>[34x]MSATASTATQPKPLEWLNRLRANPRIPLIVAGSAAVAIVVAMVLWAKTPDYRTLFSNLSDQDGGAIVAQLTQMNIPYRFANGSGAIEVPADKVHELRLRLAQQGLPKGGAVGFELLDQEKFGISQFSEQVNYQRALEGELARTIETLGPVKSARVHLAMPKPSLFVREQKSPSASVTVTLEPGRALDEGQISAVVHLVSSAVAGLPPGNVTLVDQSGHLLTQSNTSGRDLNDAQLKFANDVESRIQRRIEAILSPIVGNGNVHAQVTAQLDFANKEQTEEHYSPNGDASKATLRSRQLNISEQVGAGYPGGVPGALSNQPAPPNEAPIATPPTNQQNAQNTPQTSTSTNSNSAGPRSTQRNETSNYEVDRTIRHTKMNVGDIERLSVAVVVNYKTLADGKPLPLTADQMKQIEDLTREAMGFSDKRGDTLNVVNSPFSAVDNTGGELPFWQQQSFIDQLLAAGRWLLVLVVAWILWRKAVRPQLTRRVEEAKAAQEQAQVRQETEEAVEVRLSKDEQLQQRRANQRLGAEVMSQRIREMSDNDPRVVALVIRQWMSNDHE;>MSNLSGTDKSVILLMTIGEDRAAEVFKHLSTREVQALSTAMANVRQISNKQLTDVLSEFEQEAEQFAALNINANEYLRSVLVKALGEERASSLLEDILETRDTTSGIETLNFMEPQSAADLIRDEHPQIIATILVHLKRSQAADILALFDERLRHDVMLRIATFGGVQLAELTEVLNGLLDGQNLKRSKMGGVRTAAEIINLMKTQQEEAVITAVREFDGELAQKIIDEMFLFENLVDVDDRSIQRLLQEVDSESLLIALKGAEPPLREKFLRNMSQRAADILRDDLANRGPVRLSQVENEQKAILLIVRRLAETGEMVIGSGEDTYV[34x];>[34x]MGDSILSQAEIDALLNGDSDTKDEPTPGIASDSDIRPYDPNTQRRVV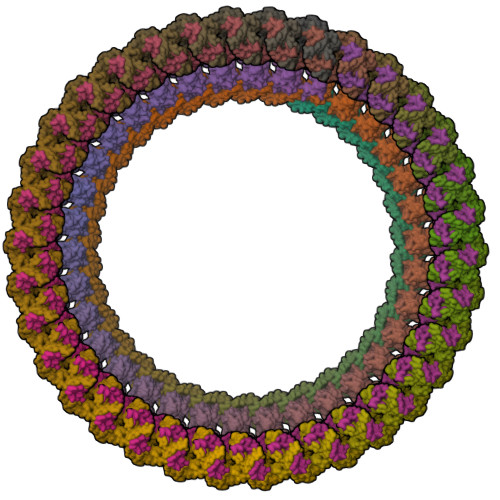RERLQALEIINERFARQFRMGLFNLLRRSPDITVGAIRIQPYHEFARNLPVPTNLNLIHLKPLRGTGLVVFSPSLVFIAVDNLFGGDGRFPTKVEGREFTHTEQRVINRMLKLALEGYSDAWKAINPLEVEYVRSEMQVKFTNITTSPNDIVVNTPFHVEIGNLTGEFNICLPFSMIEPLRELLVNPPLENSRHEDQNWRDNLVRQVQHSELELVANFADIPLRLSQILKLKPGDVLPIEKPDRIIAHVDGVPVLTSQYGTVNGQYALRVEHLINPILNSLNEEQPK;>MSDMNNPSDENTGALDDLWADALNEQKATTTKSAADAVFQQLGGGDVSGAMQDIDLIMDIPVKLTVELGRTRMTIKELLRLTQGSVVALDGLAGEPLDILINGYLIAQGEVVVVADKYGVRITDIITPSERMRRLSR[102x]10-PROPARGYL-5,8-DIDEAZAFOLIC ACID | C24 H23 N5 O6 | 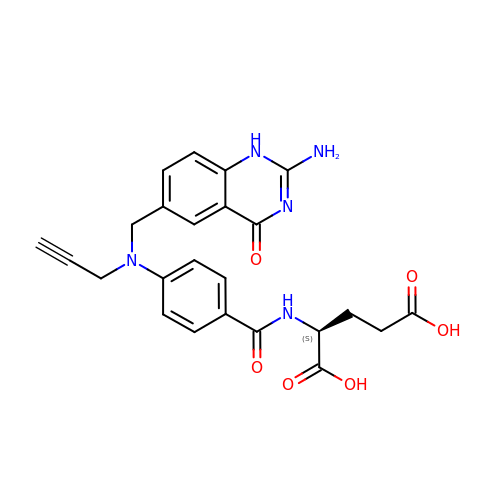LTKHPMDRMUCUEB-IBGZPJMESA-N> IVGGKVCPKGECPWQVLLLVNGAQLCGGTLINTIWVVSAAHCFDKIKNWRNLIAVLGEHDLSEHDGDEQSRRVAQVIIPSTYVPGTTNHDIALLRLHQPVV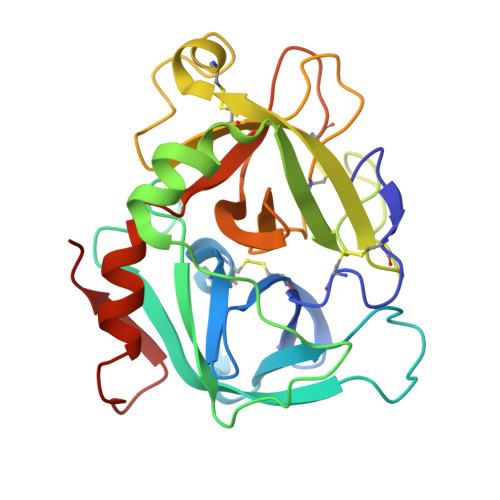LTDHVVPLCLPERTFSERTLAFVRFSLVSGWGQLLDRGATALELMVLNVPRLMTQDCEASYPGKITEYMFCAGYSDGSKDSCKGDSGGPHATHYRGTWYLTGIVSWGQGCATVGHFGVYTRVSQYIEWLQKLMRSEPRPGVLLRAPFP> DIDECDQGSPCEHNGICVNTPGSYRCNCSQGFTGPRCETNINECESHPCQNEGSCLDDPGTFRCVCMPGFTGTQCEIDIDECQSNPCLNDGTCHDKIN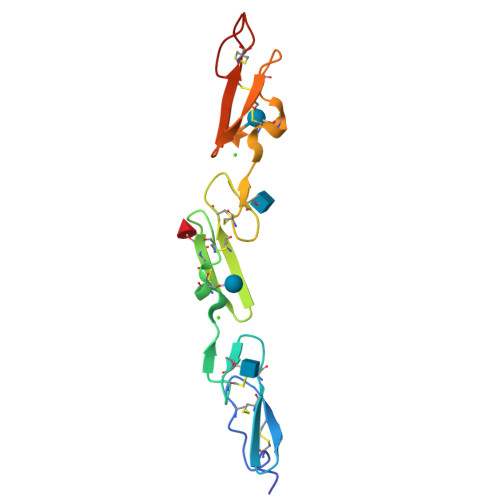GFKCSCALGFTGARCQIN> MAETREGGQSGAASILGAEAFPELLSKVPLNPQMDEDKHFNKYKWGNEPIPVNRRTGSRMNSSIYDNRNHEAVRHPWST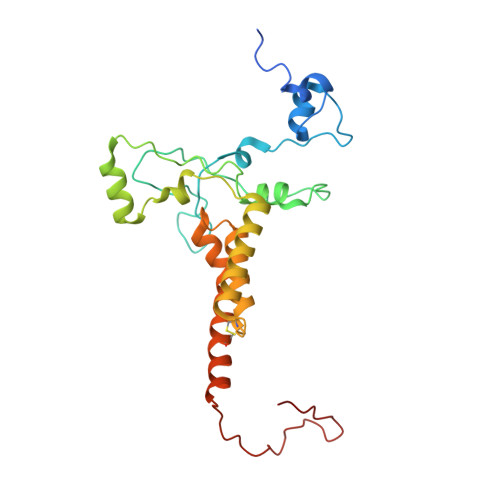DARTFHPNDNPEADRINTQYSNMVSDSFPEGGFSDAPRFSSNWERLLAYHHGLYSPEKFNSTTKTADEIRLAVNDFAAKVHADDPKNACKYLMIEEFKCLQSAQARIDPQGAATKCVKWFNEWRQCAWDQEKMVKGYNYIEDRRARKHKPYIGAPDLQYS Vactosertib | C22 H18 F N7 | 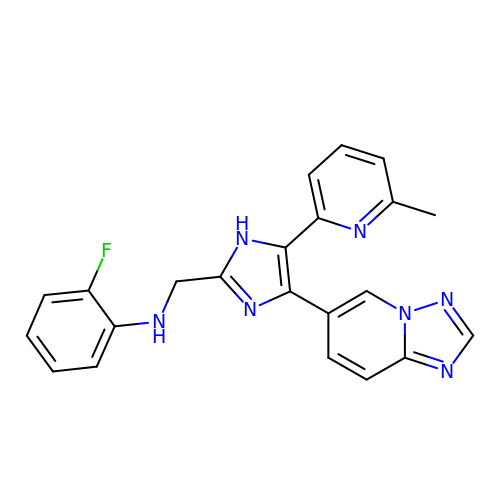FJCDSQATIJKQKA-UHFFFAOYSA-N Here we present new structural data for an IBP identified from a cold-tolerant fungus, Antarctomyces psychrotrophicus (AnpIBP). The structure of AnpIBP consists of a 45-Å-long β-helical fold with a triangular cross section. The main constituents are 6-ladder β-helical loops, which are supported by a long α-helix located along the β-helical axis. The AnpIBP uniquely binds to the water molecules that participate in the primary and secondary prism planes, which were detected as a prism ring in the FIPA experiment.

An asymmetric unit contains six AnpIBP molecules. The final model of AnpIBP shows the structural coordinates of 203 out of 216 amino acid residues. The crystal structure shows that D55, whose original residue is N55 modified with a glycan, is located at the C-terminal end of the long α-helix and is far distant from the B-face containing the IBS. Among the six AnpIBPs, half of the IBSs were covered by another protein, whereas the other half was exposed to the solvent. When we identified the water molecules whose oxygen atoms are proximal to each other within 3.5 Å to be connected with a hydrogen bond, a total of 88 water molecules were displayed on the solvent-exposed IBS. The molecules are mainly organized into polygonal arrangements similarly to those observed in Maxi, which extend over the left and right sides of the IBS in AnpIBP. There are at least 13 polygons on the IBS of AnpIBP, which are mainly located around S153 and T156. The presence of four regularly arrayed hollows was identified in the IBS of AnpIBP. The distance between the first and second hollows and between the third and fourth hollows is 4.6 Å, and that between the first and third hollows and between the second and fourth hollows is 14.7 Å. These intervals perfectly match the oxygen atom distance in the primary and secondary prism planes (4.6 and 14.7 Å) as well as that comprising the prism ring.

>HHHHHHTGLDLGAASSFGALAPQGVANAGATVINGDMGTTGTSITGFPPGLITGQLHINDDTSTQAFADSRTAFVAGQALIATVDQAGTATLGGNTFVAGVYKYDSAVGLDGVLTLDGAGDASSVWVFQLATTLVTYASSSIILTNGAKANNVFWIVGSSATLGTYSHLEGNVIANALIAAQTGATINGALLAGSAVTLDSNTVTVQNSASKLVRSAKFFKV[6x]>AAPTEAEIIASGKGKFAWPLRGDIISSFGVKGTGQRNDGLNIRAPQGTPVLSSADGEIAYAGNQVPTFGNLVLVKHADGWVTAYAHLSSTNVKMRQQVKQGEQLGTVGATGGVNEPQLHFEMRYAPTVKDKAKPVDPALVLPR[2x];>[2x]TIIETAAAPTEAEIIASGKGKFAWPLRGDIISSFGVKGTGQ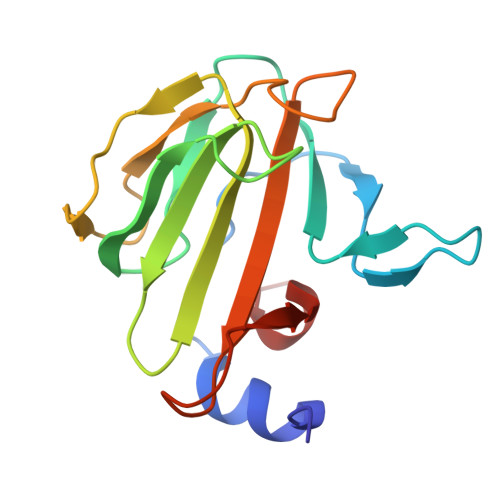RNDGLNIRAPQGTPVLSSADGEIAYAGNQVPTFGNLVLVKHADGWVTAYAHLSSTNVKMRQQVKQGEQLGTVGATGGVNEPQLHFEMRYAPTVKDKAKPVDPALVLPR>GHMSITENTSWNKEFSAEAVNGVFVLCKSSSKSCATNDLARASKEYLPASTFKIPNAIIGLETGVIKNEHQVFKWDGKPRAMKQWERDLTLRGAIQVSAVPVFQQITREVGEVRMQKYLKKFSYGNQNISGGIDKFWLEGQLRISAVNQVEFLE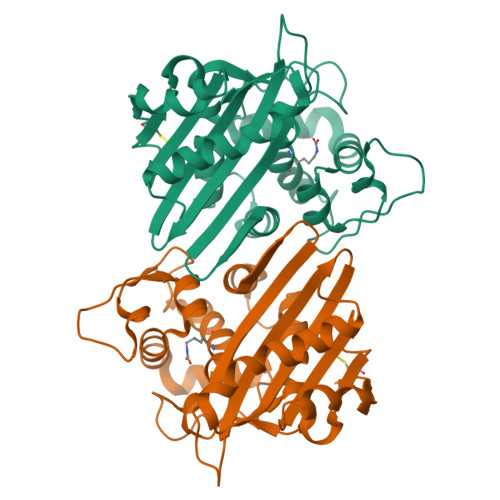SLYLNKLSASKENQLIVKEALVTEAAPEYLVHSKTGFSGVGTESNPGVAWWVGWVEKETEVYFFAFNMDIDNESKLPLRKSIPTKIMESEGIIG[2x]> AEFTSPYFGRPSLKTRAKQF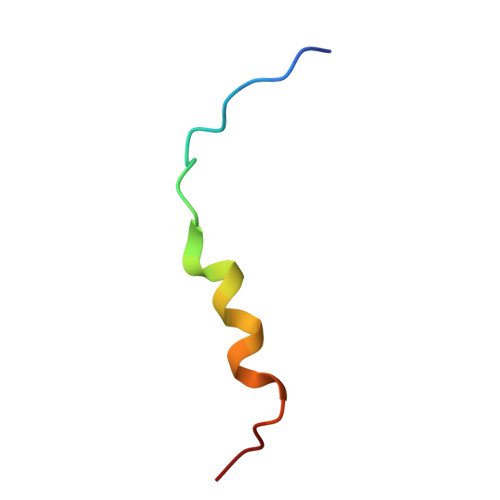EGVSSP> GSQKERLLDELTLEGVARYMQSERCRRVICLVGAGISTSAGIPDFRSPSTGLYDNLEKYHLPYPEAIFEISYFKKHPEPFFALAKELYPGQFKPTICHYFMRLLKDKGLLLRCYTQNIDTLERIAGLEQEDLVEAHGTFYTSHCVSASCRHEYPLSWMKEKIFSEVTPKCEDC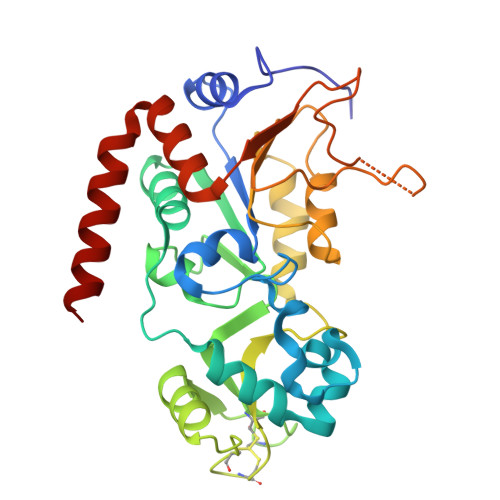QSLVKPDIVFFGESLPARFFSCMQSDFLKVDLLLVMGTSLQVQPFASLISKAPLSTPRLLINKEKAGQSDPFLGMIMGLGGGMDFDSKKAYRDVAWLGECDQGCLALAELLGWKKELEDLVRREHASIDAQ> GAMEAMQKNELNSKIPIIFGLINSYQIHNLLEQHNAKTKESKAVFLIRDSSTYPGLLTISYYCQEQDIVKHIRFGLTDKGWKTAPKPPHEPLKSD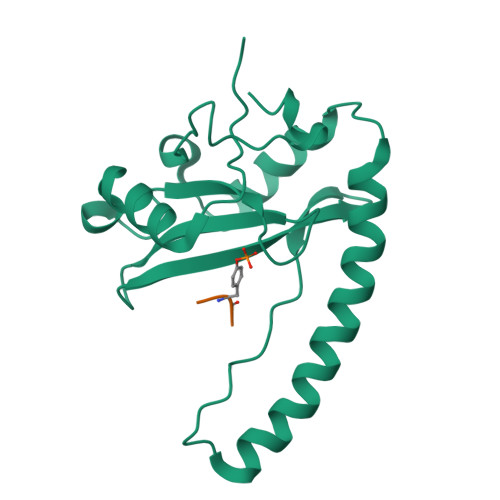SPEIKEKYTLDKIKFERKMKQFINTAKKLFEQHIRAESFKTLIMELKIHEFNLEGLIKPTRSQASQEKHFTDYV;> YFTYDPYSEEDPD> GSHMSRKIRDLIESKRFQNVITAIIVLNGAVLGLLTDTTLSASSQNLLERVDQLCLTIFIVEISLKIYAYGVRGFFRSGWNLFDFVIVAIALMPAQGSLSVLRTFRIFRVMRLVSVIPTMRRVVQGMLLALPGVGSVAALLTVVFYIAAVMATNLYGATFPEWFGDLSKSLYTLFQVMTLESWSMGIVRPVMNVHPNAWVFFIPFIMLTTFTVLNLFIGICVDAMAITKEQEEEAKTGHHQEPISQTLLHLGDRLDRIEKQLAQNNELLQRQQPQKK

Prokaryotic sodium channels, in contrast, are true tetrameric structures, composed of four identical subunits, each one equivalent to a single eukaryotic region. Both eukaryotic and prokaryotic Navs consist of voltage sensor (VS) and pore domains, which are responsible for regulation and ion-translocation functions, respectively, and C-terminal domains (CTDs), which appear in both cases to have regulatory functions, albeit of quite different natures and structures. Prokaryotic orthologues exhibit approximately 25–30% sequence identity with human Navs and several have been shown to have sodium ion translocation activity and one (NavMs from Magnetococcus marinus) has been shown to be blocked by human sodium channel blockers with similar affinities and kinetics as the human Nav1.1 isoform3, thus indicating the structure/function similarities of eukaryotic and prokaryotic Nav orthologues.

In this study, the high-resolution crystal structure of a complete voltage-gated sodium channel (with crystals formed under zero potential conditions consistent with an open-channel state) has been determined. The structure displays an activated VS domain conformation, three sodium ions present in its open selectivity filter, and an open intracellular pore gate formed from the S6 transmembrane helices leading into a regulatory CTD. It has revealed the nature of an interaction domain that forms the basis for understanding the opening and closing of the intracellular gate, and indicated a set of residues essential for enabling the open conformation, including signature residues that are conserved across prokaryotic and eukaryotic sodium channels. The present structure is the only complete crystal structure of any sodium channel determined to date. It is also the only sodium channel with an activated VS and a pore gate sufficiently wide to enable the passage of sodium ions, both features expected for an ‘open' state channel, and as such it is likely to form the basis for new molecular dynamics simulations of ion translocation.> ASAKLPGDFGPPRGEPIHAVLTSPPLVPPPVNRTYPAKVIVELEVVEKEMQISEGVSYTFWTFGGTVPGSFIRVRQGDTVEFHLKNHPSSKMPHNIDLHGVTGPGGGAASSFTAPGHESQFTFKALNEGIYVYHCATAPVGMHIANGMYGLILVEPPEGLPKVDHEYYVMQGDFYTAGKYREKGLQPFDMEKAIDERPSYVLFNGAEGALTGDKALHAKVGETVRIFVGNGGPNLVSSFHVIGAIFDQVRYEGGTNVQKNVQTTLIPAGGAAVVKFTARVPGSYVLVDHSIFRAFNKGAM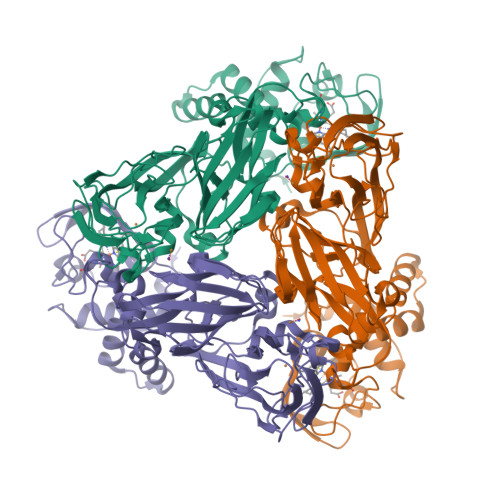AILKIDGAENKLVYSGKELDSVYLGDRAAPNMSAVTKATQASVSGTLTVQDQVQAGRALFAGTCSVCHQGNGAGLPGVFPPLAKSDFLAADPKRAMNIVLHGLNGKIKVNGQEYDSVMPPMTQLNDDEVANILTYVLNSWDNPGGRVSAEDVKKVRAQPAPAKAVAEH>[2x]DTKEQRILRYVQQNAKPGDPQSVLEAIDTYCTQKEWAMNVGDAKGQIMDAVIREYSPSLVLELGAYCGYSAVRMARLLQPGARLLTMEMNPDYAAITQQMLNFAGLQDKVTILNGASQDLIPQLKKKYDVDTLDMVFLDHWKDRYLPDTLLLEKCGLLRKGTVLLADNVIVPGTPDFLAYVRGSSSFECTHYSSYLELMKVVDGLEKAIYQGP

One example where the lack of enzyme regioselectivity limits potential commercial productivity is the engineered biosynthesis of the flavor and fragrance agent vanillin 2 a.3 Catechol‐O‐methyltransferase (COMT) has been used to methylate 3,4‐dihydroxybenzaldehyde (DHBAL, 1 a) and 3,4‐dihydroxybenzoic acid (DHBA, 1 b) in engineered strains of Escherichia coli and fission yeast for the production of vanillin 2 a from glucose. However, the lack of regioselectivity of COMT results in a mixture of 2 a and the undesired para‐methylated isovanillin 3 a, which are difficult to separate. Structural and mechanistic information suggest that the regioselectivity of COMT can be attributed to the concerted action of a “hydrophobic wall” found in the active site of the enzyme, and the substrate properties. The orientation of the R group in the active site determines whether the meta‐ or para‐hydroxy group is methylated.

The Y200 mutants generally showed increased re values in favor of the meta product with all substrates, with Y200L exhibiting the greatest meta‐selectivity with 1 a–d whilst retaining relative activity similar to that of the WT with 1 a and 1 d. The X‐ray crystal structures of dimeric Y200L and WT COMT revealed that a key residue (E199) had been flipped out of the active site. We rationalize that in the WT monomeric enzyme, E199 can form a hydrogen bond with the aldehyde group of 1 a, thereby leading to some para‐methylation, whereas in dimeric Y200L and WT COMT the absence of E199 from the active site results in the aldehyde group orientating towards the solvent, thereby leading to meta‐methylation. In contrast, both oligomeric forms of Y200L showed high re values with 1 a (ca +90 %). However, the re value for Y200L monomer (ca. +90 %) suggests that in the absence of dimerization, the Y200L mutation alone is sufficient to cause loss of E199 interaction with the substrate. Since monomeric Y200L is as regioselective as the dimeric forms (ca. +90 % re), we suggest, based on the structural data for the Y200L and WT dimers and the regioselectivity assay data for both oligomeric forms, that loss of para‐methylation is largely due to movement of E199 out of the active site, as a consequence either of mutagenesis (Y200L) or protein dimerization and domain swapping (WT). Active‐site modifications thus appear to cause significant shifts in regioselectivity independently of the enzyme oligomeric state. Finally, we demonstrated potential applications for our improved COMT variants by regioselectively alkylating 1 a by using ethyl, allyl, and benzyl AdoMet analogues generated enzymatically or synthetically.11 Products 4 a–c were obtained with re values of approximately +90 % with Y200L compared to +33–45 % with WT COMT.> AMKKILSFDIDNTLN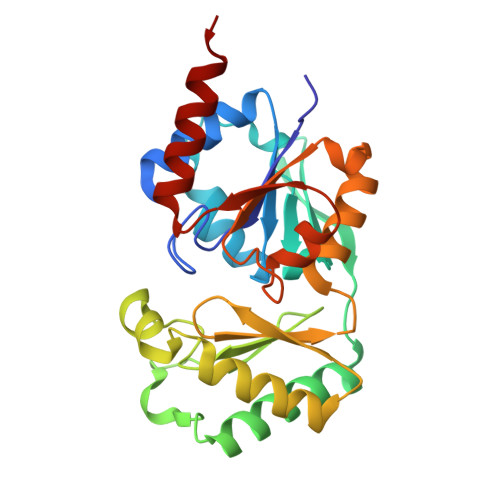EPKMPIFPEMAELLATLSQKYIIAPISGQKYDQFLIQIINNLPESANLDNFHLFVAQGTQYYAHKAGEWKQVFNYALTDEQANAIMGALEKAAKELGHWDESVLLPGDEINENRESMIAYSAIGQKAGVEAKQAWDPDMTKRNEIAKLASQYAPEFEFEVAGTTTINGFVPGQNKEFGMNHLMEELNVTKEEILYFGDMTQPGGNDYPVVQMGIETITVRDWKETAAILKAIIAMEEA> MHHHHHHMLSVDDCFGMGRSAYNEGDYYHTVLWMEQVLKQLDAGEEATTTKSQVLDYLSYAVFQLGDLHRALELTR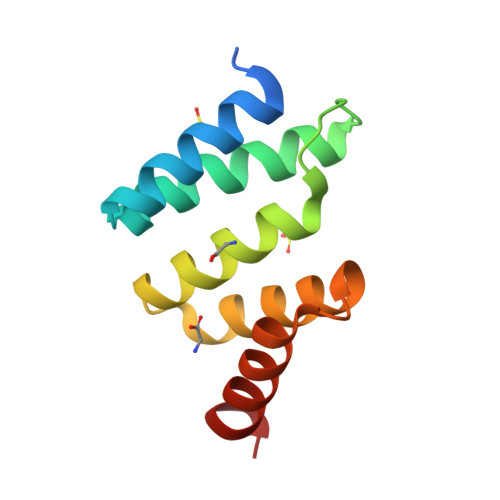RLLSLDPSHERAGGNLRYFEQLLEEE> XALETLRRV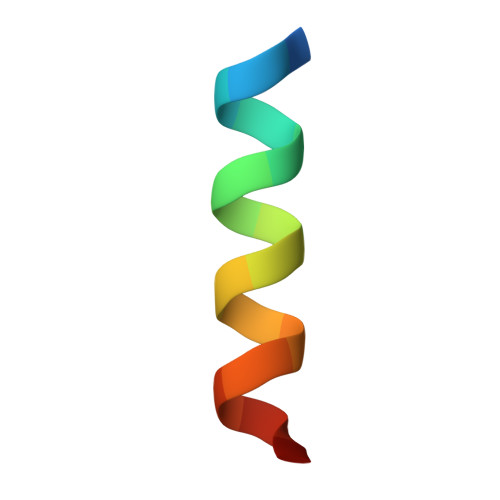GDGVQRNHX>MAHHHHHHVGTGSNDDDDKSPDPTHNKPLPENVKYGIVLDAGSSHTNLYIYKWPAEKENDTGVVQQLEECQVKGPGISKYAQKTDEIAAYLAECMKMSTERIPASKQHQTPVYLGATAGMRLLRMESKQSADEVLAAVSRSLKSYPFDFQGAKIITGQEEGAYGWITINYLLGRFKTPGGSTFGALDLGGSSTQITFVPLNSTLEAPETSLQFRLYGTDYTVYTHSFLCYGKDQALWQKLAQDIQVSSGGILKDPCFYPGYKKVVNVSELYGTPCTKRFEKKLPFNQFQVQGTGDYEQCHQSILKIFNNSHCPYSQCAFNGVFLPPLQGSFGAFSAFYFVMDFFKKMANDSVSSQEKMTEITKNFCSKPWEEVKASYPTVKEKYL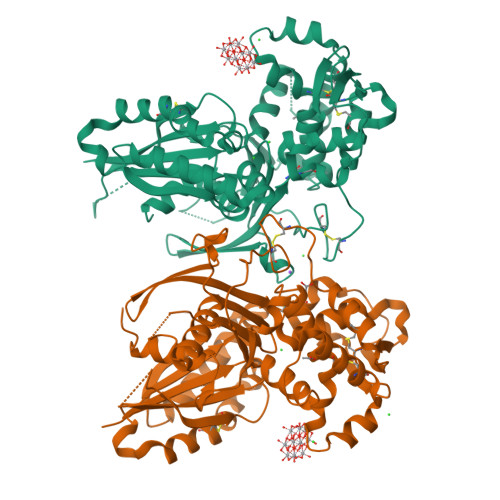SEYCFSGTYILSLLLQGYNFTGTSWDQIHFMGKIKDSNAGWTLGYMLNLTNMIPAEQPLSPPLPHST[4x]> MKVVNLKQAILQAWKERWSDYQWAINMKKFFPKGATWDILNLADALLEQAMIGPSPNPLILSYLKYAISSQMVSYSSVLTAISKFDDFSRDLCVQALLDIMDMFCDRLSCHGKAEECIGLCRALLSALHWLLRCTAASAERLREGLEAGTPAAGEKQLAMCLQRLEKTLSSTKNRALLHIAKLEEASSWTAIEHSLLKLGEILANLSNPQLRSQAEQCGTLIRSIPTMLSVHAEQMHKTGFPTVHAVILLEGTMNLTGETQSLVEQLTMVKRMQHIPTPLFVLEIWKACFVGLIESPEGTEELKWTAFTFLKIPQVLVKLKKYSHGDKDFTEDVNCAFEFLLKLTPLLDKADQRCNCDCTNFLLQECGKQGLLSEASVNNLMAKRKADREHAPQQKSGENANIQPNIQLILRAEPTVTNILKTMDADHSKSPEGLLGVLGHMLSGKSLDLLLAAAAATGKLKSFARKFINLNEFTTYGSEESTKPASVRALLFDISFLMLCHVAQTYGSEVILSESRTGAEVPFFETWMQTCMPEEGKILNPDHPCFRPDSTKVESLVALL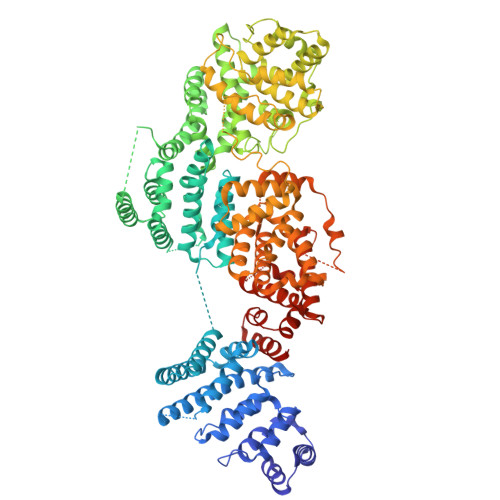NNSSEMKLVQMKWHEACLSISAAILEILNAWENGVLAFESIQKITDNIKGKVCSLAVCAVAWLVAHVRMLGLDEREKSLQMIRQLAGPLFSENTLQFYNERVVIMNSILERMCADVLQQTATQIKFPSTGVDTMPYWNLLPPKRPIKEVLTDIFAKVLEKGWVDSRSIHIFDTLLHMGGVYWFCNNLIKELLKETRKEHTLRAVELLYSIFCLDMQQVTLVLLGHILPGLLTDSSKWHSLMDPPGTALAKLAVWCALSSYSSHKGQASTRQKKRHREDIEDYISLFPLDDVQPSKLMRLLSSNEDDANILSSPTDRSMSSSLSASQLHTVNMRDPLNRVLANLFLLISSILGSRTAGPHTQFVQWFMEECVDCLEQGGRGSVLQFMPFTTVSELVKVSAMSSPKVVLAITDLSLPLGRQVAAKAIAAL Aminoacyl-tRNA synthetases (ARSs) catalyze the ligation of each amino acid to the 3’ hydroxyl group of the cognate tRNA and thereby establish the genetic code for protein synthesis. ARSs assemble into a multi-synthetase complex (MSC), which is comprised of nine ARSs (arginyl- (RARS1), aspartyl- (DARS1), glutaminyl- (QARS1), glutamyl-proryl- (EPRS1), isoleucyl- (IARS1), leucyl- (LARS1), lysyl- (KARS1), and methionyl-tRNA synthetase 1 (MARS1)) and three auxiliary proteins (ARS-interacting multifunctional proteins, AIMP1 (p43), AIMP2 (p38), and AIMP3 (p18)) in vertebrates. IARS1 is one of the least characterized ARSs in the MSC. It is a class 1a ARS and has an UNE-I domain at its C-terminal end that is formed by tandem ~90 residue repeats. The overall structure of GgEARS1 consists of an N-terminal catalytic domain (acceptor end-binding and dinucleotide-binding domains) and C-terminal anticodon-binding domain (proximal β-barrel (Pβ) and distal β-barrel (Dβ) domains).

While we could not improve the size and quality of the crystals, we determined the structure of the GgEARS1–IARS1 complex at 2.4 Å resolution using the Pohang Advanced Light Source X-ray free electron laser (PAL-XFEL). The first β-grasp domain corresponds to the KH domain, whereas the second and third β-grasp domains most resemble Ub or the UBX domain with a rms deviation value of 1.8 and 2.0 Å, respectively, for 76 Cα residues, which we termed UBX1 and UBX2. Upon packing, a wide groove with a width of 15 Å, height of 10 Å, and depth of 11 Å is formed between the first helices of UBX1 and UBX2. The UBX1 and UBX2 domains both directly interact with EARS1 via the groove between the inter-helices at the obscured face. A total of 2429 Å2 of surface area becomes buried upon complex formation. The first interface is formed between UBX2 and the helical subdomain (stem-binding domain) of EARS1. The second interface is defined between the two UBX domains and the extended hairpin loop (22 Å long, residues Tyr684 to Pro696) of the EARS1 Pβ domain. At the tip of the hairpin loop, two conserved Ser (Ser688 and Ser691) and one Tyr (Tyr690) residues are present. Although Ser691 is not involved in the direct interaction with the UBX domains, Ser688 makes contact with Glu1216 of UBX2, whereas Tyr690 interacts with Leu1198 and Asn1206. While mutation of Ser688 or Ser691 to glutamate retained the interaction of EARS1 with IARS1, simultaneous mutation of both residues dissociated IARS1 from EARS1.

> MATEKKADVGKFVELPGAEMGKVIVRFPPEASGYLHIGHAKAALLNQHYQVNFKGKLIMRFDDTNPEKEKEDFEKVILEDVAMLHIKPDQFTYTSDHFETIMKYAEQLIQEGKAYVDDTPAEQMKAEREQRMESKHRNNCVNKNLQMWEEMKKGTEYGQTCCLRAKIDMNSNNGCMRDPTLYRCKNQPHPRTGTTYKVYPTYDFACPIVDSIEGVTHALRTTEYHDRDEQFYWIIEALGIRKPYIWEYSRLNLNNTVLSKRKLMWFVNEGLVDGWDDPRFPTVRGVLRRGMTVEGLKQFIAAQGSSRSVVNMEWDKIWSFNKKVIDPVAPRYTALLKDAVVPVNVPEAQEEMKEVAKHPKNADVGLKPVWYGSKVLIEGADAETLTEGEVVTFINWGNIIITKLNRNSSGKIVSIDTKLNLDNKDFKKTTKITWLAETPRAPLIPTVCVNYEHLITKPVLGKDEDFKQYINRNSKQEELMLGDPCLKDLKKGDIIQLQRRGFFICDQPYEPVSPYSCKEAPCILIYIPDGH;> HSDAQVLVLLDVTPDQSMVDEGVAREVINRIQKLRKKRNLVPTDEITVYYRSHPEGDYLDTVIKEHTDFIFATIKAALKPYPVPTSKEVLIQETTQLKGSELEITLVRGGLCERVGPACSYVNLKVCVNGTEQDGVLLLENPKGDNTLNLTGLVDAVSCIFGLKNSKLTVFNGKTELINKTDLLSLSGKTLHVTTGSAPALINSPDALLCQYINLQLVNAKPQECQKGTVGTLLMENPVGQNGLTYHGLLHETAKVFGLRSRRLKLFLDEAETQEITKDISMKNLNMKTVYVSVIPTTAEC>[3x]MKLFLILLVLPLASCFFTCNSNANLSMLQLGVPDNSSTIVTGLLPTHWFCANQSTSVYSANGFFYIDVGNHRSAFALHTGYYDANQYYIYVTNEIGLNASVTLKICKFSRNTTFDFLSNASSSFDCIVNLLFTEQLGAPLGITISGETVRLHLYNVTRTFYVPAAYKLTKLSVKCYFNYSCVFSVVNATVTVNVTTHNGRVVNYTVCDDCNGYTDNIFSVQQDGRIPNGFPFNNWFLLTNGSTLVDGVSRLYQPLRLTCLWPVPGLKSSTGFVYFNATGSDVNCNGYQHNSVVDVMRYNLNFSANSLDNLKSGVIVFKTLQYDVLFYCSNSSSGVLDTTIPFGPSSQPYYCFINSTINTTHVSTFVGILPPTVREIVVARTGQFYINGFKYFDLGFIEAVNFNVTTASATDFWTVAFATFVDVLVNVSATNIQNLLYCDSPFEKLQCEHLQFGLQDGFYSANFLDDNVLPETYVALPIYYQHTDINFTATASFGGSCYVCKPHQVNISLNGNTSVCVRTSHFSIRYIYNRVKSGSPGDSSWHIYLKSGTCPFSFSKLNNFQKFKTICFSTVEVPGSCNFP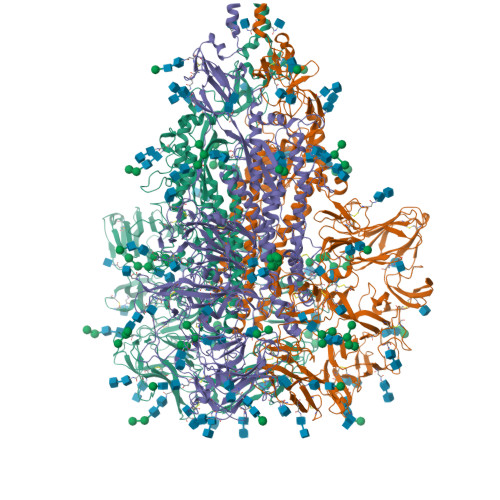LEATWHYTSYTIVGALYVTWSEGNSITGVPYPVSGIREFSNLVLNNCTKYNIYDYVGTGIIRSSNQSLAGGITYVSNSGNLLGFKNVSTGNIFIVTPCNQPDQVAVYQQSIIGAMTAVNESRYGLQNLLQLPNFYYVSNGGNNCTTAVMTYSNFGICADGSLIPVRPRNSSDNGISAIITANLSIPSNWTTSVQVEYLQITSTPIVVDCATYVCNGNPRCKNLLKQYTSACKTIEDALRLSAHLETNDVSSMLTFDSNAFSLANVTSFGDYNLSSVLPQRNIRSSRIAGRSALEDLLFSKVVTSGLGTVDVDYKSCTKGLSIADLACAQYYNGIMVLPGVADAERMAMYTGSLIGGMVLGGLTSAAAIPFSLALQARLNYVALQTDVLQENQKILAASFNKAINNIVASFSSVNDAITQTAEAIHTVTIALNKIQDVVNQQGSALNHLTSQLRHNFQAISNSIQAIYDRLDSIQADQQVDRLITGRLAALNAFVSQVLNKYTEVRGSRRLAQQKINECVKSQSNRYGFCGNGTHIFSIVNSAPDGLLFLHTVLLPTDYKNVKAWSGICVDGIYGYVLRQPNLVLYSDNGVFRVTSRVMFQPRLPVLSDFVQIYNCNVTFVNISRVELHTVIPDYVDVNKTLQEFAQNLPKYVKPNFDLTPFNLTYLNLSSELKQLEAKTASLFQTTVELQGLIDQINSTYVDLKLLNRFENYIKWPWWVWLIISVVFVVLLSLLVFCCLSTGCCGCCNCLTSSMRGCCDCGSTKLPYYEFEKVHVQ> SNAIPIFLSVLQSIEPEVVYAGYDNTQPDTSASLLTSLNELGERQLVRVVKWAKALPG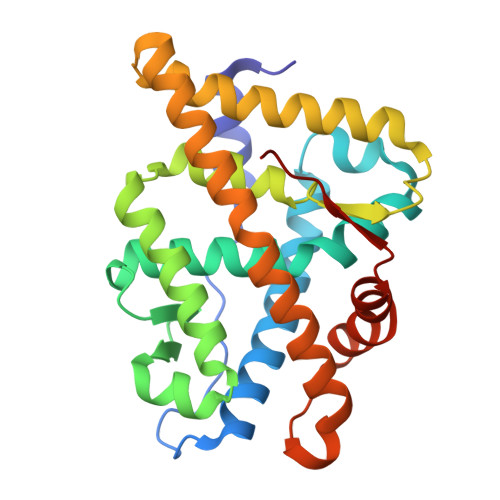FRNLHVDDQMTLIQYSWMGVMVFAMGWRSYKNVNSRMLYFAPDLVFNEQRMQKSTMYNLCVRMRHLSQEFVWLQVTQEEFLCMKALLLFSIIPVEGLKNQKYFDELRMNYIKELDRVISFQGKNPTSSSQRFYQLTKLLDSLQPIVRKLHQFTFDLFVQSQSLSVEFPEMMSEIISAQVPKILAGMVKPLLFHKQ Member 6 of the vanilloid family of transient receptor potential channels, TRPV6, is a master regulator of organismal Ca2+ homeostasis. TRPV6 acts as the major dietary calcium uptake channel in the human gut3, and as such, this channel remains constitutively active, while its activity is regulated positively by membrane lipids such as phosphatidylinositol 4,5-bisphosphate (PIP2)4–6 and negatively by Mg2+ ions. It consists of four subunits and features a transmembrane domain (TMD) that houses the central ion channel pore, along with an intracellular skirt primarily composed of ankyrin repeat domains interconnected by three-stranded β-sheets, N-terminal helices, and C-terminal hooks. The TMD includes six transmembrane helices (S1–S6) and a re-entrant pore loop (P-loop) between S5 and S6.

To avoid possible interference of Mg2+ inhibition with CaM-mediated inactivation, we utilized the C-terminally truncated hTRPV6 construct (hTRPV6-CtD) that lacks the CaM-binding site and has been extensively used in the previous structural studies of TRPV6 as its function is identical to wild-type channels with the only exception of lacking CaM-induced inactivation. Single-particle cryo-EM analysis of purified, lipid nanodisc-reconstituted hTRPV6-CtD, henceforth referred to as TRPV6, in the presence of Mg2+ yielded a 2.97-Å resolution hTRPV6Mg structure. Besides the densities for a magnesium ion tightly bound inside the channel selectivity filter and annular lipids surrounding the TMD, commonly observed in the previously published TRPV6 structures, we observed four spherical densities, one per hTRPV6Mg subunit, around the intracellular entrance to the ion channel pore. Each Mg2+ ion in these putative Mg2+ binding sites is coordinated by the backbone carbonyl of K484 in S5 and carboxyl groups of D489 in S5 and D580 in S6. The pore in the hTRPV6Mg structure has two narrow constrictions, one at the selectivity filter, formed by the calcium-coordinating side chains of D542, and the second at the gate region, formed by the hydrophobic side chains of L574 and M578. This pore conformation is typical for the closed-state TRPV6 structures and different from the open, apo-state structures. Typical for the open-to-closed transition during TRPV6 gating, the narrowing of the hTRPV6Mg pore is accompanied by a ~100-degree rotation of the S6 intracellular portion. During this rotation, S6, which has a π-bulge following the gating hinge alanine A566 in hTRPV6Open, becomes entirely α-helical in hTRPV6Mg. By recruiting D489 and D580 into coordination, Mg2+ ions, therefore, disfavor the interaction between D489 and T581 and stabilize the closed state, accordingly. Mg2+ binding to the D489-D580 site prevents separation of these residues and rotation of the lower part of S6 that accompanies channel opening, thus locking the channel in the closed state.

>[4x]ESWAQSRDEQNLLQQKRIWESPLLLAAKDNDVQALNKLLKYEDCKVHQRGAMGETALHIAALYDNLEAAMVLMEAAPELVFEPMTSELYEGQTALHIAVVNQNMNLVRALLARRASVSARATGTAFRRSPCNLIYFGEHPLSFAACVNSEEIVRLLIEHGADIRAQDSLGNTVLHILILQPNKTFACQMYNLLLSYDRHGDHLQPLDLVPNHQGLTPFKLAGVEGNTVMFQHLMQKRKHTQWTYGPLTSTLYDLTEIDSSGDEQSLLELIITTKKREARQILDQTPVKELVSLKWKRYGRPYFCMLGAIYLLYIICFTMCCIYRPLKPRTNNRTSPRDNTLLQQKLLQEAYMTPKDDIRLVGELVTVIGAIIILLVEVPDIFRMGVTRFFGQTILGGPFHVLIITYAFMVLVTMVMRLISASGEVVPMSFALVLGWCNVMYFARGFQMLGPFTIMIQKMIFGDLMRFCWLMAVVILGFASAFYIIFQTEDPEELGHFYDYPMALFSTFELFLTIIDGPANYNVDLPFMYSITYAAFAIIATLLMLNLLIAMMGDTHWRVAHERDELWRAQIVATTVMLERKLPRCLWPRSGICGREYGLGDRWFLRVEDRQD> MKSKKILIVGAGFSGAVIGRQLAEKGHQVHIIDQRDHIGGNSYDARDSETNVMVHVYGPHIFHTDNETVWNYVNKHAEMMPYVNRVKATVNGQVFSLPINLHTINQFFSKTCSPDEARALIAEKGDSTIADPQTFEEEALRFIGKELYEAFFKGYTIKQWGMQPSELPASILKRLPVRFNYDDNYFNHKFQGMPKCGYTQMIKSILNHENIKVDLQREFIVEERTHYDHVFYSGPLDAFYGYQYGRLGYRTLDFKKFTYQGDYQGCAVMNYCSVDVPYTRITEHKYFSPWEQHDGSVCYKEYSRACEENDIPYYPIRQMGEMALLEKY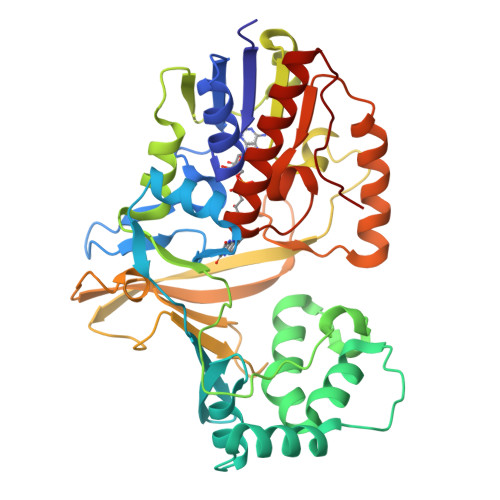LSLAENETNITFVGRLGTYRYLDMDVTIAEALKTAEVYLNSLTENQPMPVFTVSVR> GPHMASSSGNDDDLTIPRAAINKMIKETLPNVRVANDARELVVNCCTEFIHLISSEANEICNKSEKKTISPEHVIQALESLGFGSYISEVKEVLQECKTVALKRRKASSRLENLGIPEEELLRQQQELFAKARQQQAELAQQEWLQMQQAAQ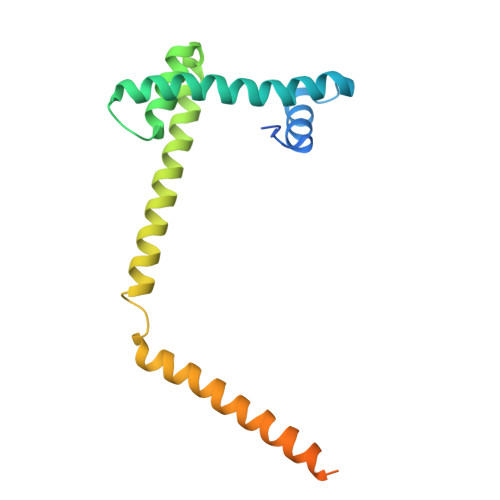QAQLAAASASASNQAGSSQDEEDDDDI>[2x]MARIIVVTSGKGGVGKTTSSAAIATGLAQKGKKTVVIDFAIGLRNLDLIMGCERRVVYDFVN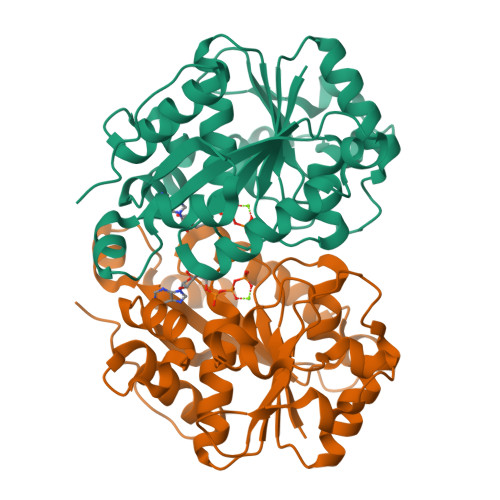VIQGDATLNQALIKDKRTENLYILPASQTRDKDALTREGVAKVLDDLKAMDFEFIVCDSPAGIETGALMALYFADEAIITTNPEVSSVRDSDRILGILASKSRRAENGEEPIKEHLLLTRYNPGRVSRGDMLSMEDVLEILRIKLVGVIPEDQSVLRASNQGEPVILDINADAGKAYADTVERLLGEERPFRFIEEEK> MMIVYKGEKMQFIRVNTL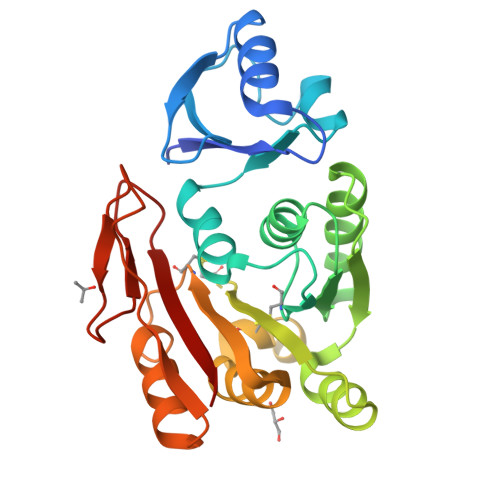KINPEVLKKRLENKGVVLEKTFLDYAFEVKKSPFSIGSTPEYLFGYYMPQSISSMIPPIVLNPREDDFILDMCAAPGGKTTHLAQLMKNKGTIVAVEISKTRTKALKSNINRMGVLNTIIINADMRKYKDYLLKNEIFFDKILLDAPCSGNIIKDKNRNVSEEDIKYCSLRQKELIDIGIDLLKKDGELVYSTCSMEVEENEEVIKYILQKRNDVELIIIKANEFKGINIKEGYIKGTLRVFPPNEPFFIAKLRKI>MASISSLGVGSNLPLDQLLTDLTKNEKGRLTPITKQQSANSAKLTAYGTLKSALEKFQTANTALNKADLFKSTVASSTTEDLKVSTTAGACAGTYKINVTQLAAAQSLATKTTFATTKEQLGDTSVTSRTIKIEQPGRKEPLEIKLDKGDTSMEAIRDAINDADSGICASIVKVKENEFQLVLTANSGTDNTMKITVEGDTKLNDLLAYDSTTNTGNMQELVKAENAKLNVNGIDIERQSNTVTDAPQGITLTLTKKVTDATVTVTKDDTKAKEAIKSWVDAYNSLVDT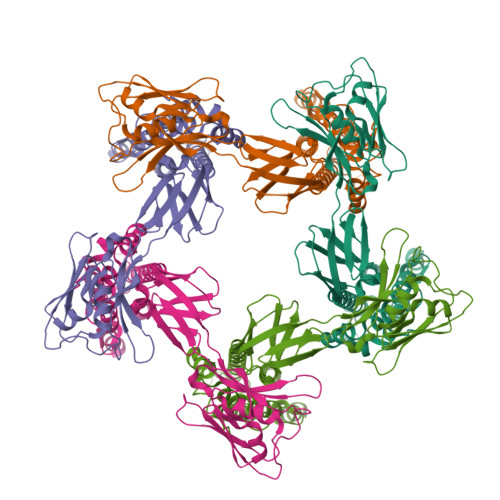FSSLTKYTAVEPGEEASDKNGALLGDSVVRTIQTGIRAQFANSGSNSAFKTMAEIGITQDGTSGKLKIDDDKLTKVLKDNTAAARELLVGDGKETGITTKIATEVKSYLADDGIIDNAQDNVNATLKSLTKQYLSVSNSIDETVARYKAQFTQLDTMMSKLNNTSSYLTQQFTAMNKS[5x]We assessed the performance of these methods in the identification of sulfur hydrogen bonds within the active site of the enzyme Alkyl hydroperoxide reductase E (AhpE) from Mycobacterium tuberculosis. To test our approach on structural coordinated atoms in space, we used the active site environment of the peroxidatic sulfur of peroxiredoxin AhpE, a single cysteine enzyme. AhpE reduces H2O2 to water but no H2O2 is present in the active site of the AhpE structures. Method 3, however, only finds the interaction with the water molecule, not the Arg116. It is predicted that stabilization of the Cys45 thiolate by Arg116 will promote its nucleophilic character, so that this Cys represents a catalytically active state of the enzyme.

To improve protein stability during MD simulations, we realized that a re-refinement of the models of the AhpE structure was needed (see supplementary). After this re-refinement operation, we repeated the simulation with the newly refined structure for chain A and found that after 30 ns the helix α2 remained intact. Importantly, a gauche minus conformation was found for the peroxydatic Cys45 in the active site of chain A after re-refinement, which is in line with the conformation reported for most of peroxiredoxins.

>KVPRGSHMLNVGATAPDFTLRDQNQQLVTLRGYRGAKNVLLVFFPLAFTGICQGELDQLRDHLPEFENDDSAALAISVGPPPTHKIWATQSGFTFPLLSDFWPHGAVSQAYGVFNEQAGIANRGTFVVDRSGIIRFAEMKQPGEVRDQRLWTDALAALT[2x]> VVQRLFQVKGRRVVRATEVPVSWESFNNGDCFILDLGNNIHQWCGSNSNRYERLKATQVSKG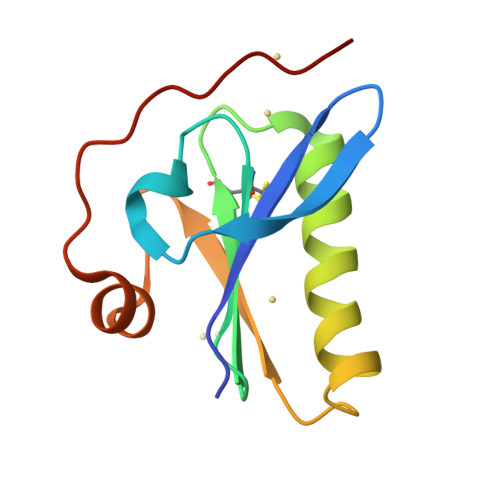IRDNERSGRARVHVSEEGTEPEAMLQVLGPKPALPAGTEDTA> ACDYTCGSNCYSSSDVSTAQAAGYKLHEDGETVGS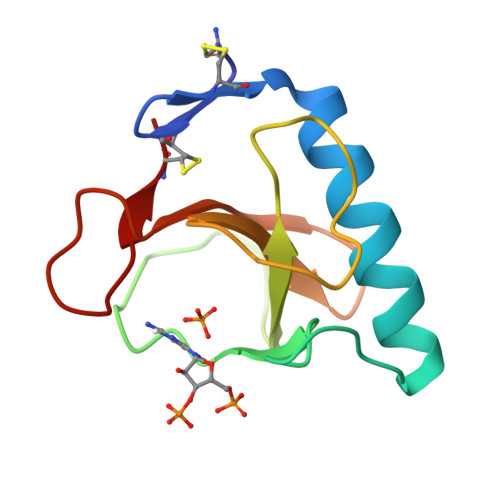NSYPHKYNNYEGFDFSVSSPYYEWPILSSGDVYSGGSPGADRVVFNENNQLAGVITHTGASGNNFVECT>[2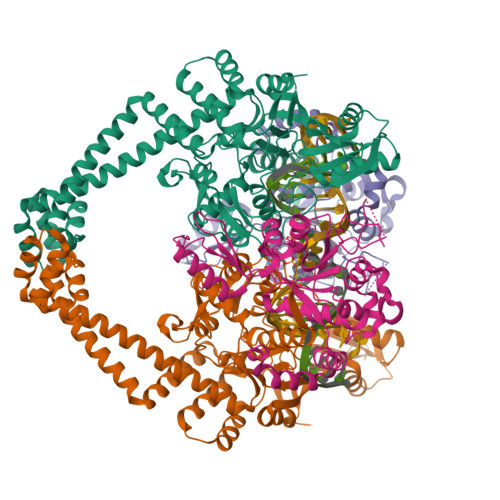x]TDTTLPPDDSLDRIEPVDIEQEMQRSYIDYAMSVIVGRALPEVRDGLKPVHRRVLYAMFDSGFRPDRSHAKSARSVAETMGNYHPHGDASIYDSLVRMAQPWSLRYPLVDGQGNFGSPGNDPPAAMRYTEARLTPLAMEMLREIDEETVDFIPNYDGRVQEPTVLPSRFPNLLANGSGGIAVGMATNIPPHNLRELADAVFWALENHDADEEETLAAVMGRVKGPDFPTAGLIVGSQGTADAYKTGRGSIRMRGVVEVEEDSRGRTSLVITELPYQVNHDNFITSIAEQVRDGKLAGISNIEDQSSDRVGLRIVIEIKRDAVAKVVINNLYKHTQLQTSFGANMLAIVDGVPRTLRLDQLIRYYVDHQLDVIVRRTTYRLRKANERAHILRGLVKALDALDEVIALIRASETVDIARAGLIELLDIDEIQAQAILDMQLRRLAALERQRIIDDLAKIEAEIADLEDILAKPERQRGIVRDELAEIVDRHGDDRRTRIIAIGSG;>SNALVRRKSATDIGGLPGKLADCRSTDPRKSELYVVEGDSAGGSAKSGRDSMFQAILPLRGKIINVEKARIDRVLKNTEVQAIITALGTGIHDEFDIGKLRYHKIVLMADADVDGQHISTLLLTLLFRFMRPLIENGHVFLAQPPLYKLKWQRSDPEFAYSDRERDGLLEAGLKAGKKINKEDGIQRYKGLGEMDAKELWETTMDPSVRVLRQVTLDDAAAADELFSILMGEDVDARRSFITRNAKDVRFLDV[2x]To neutralize chemokines, ticks secrete small cysteine-rich chemokine-binding proteins in their saliva with no homologues in mammals, termed Evasins. In contrast to the highly selective Evasin-1, its homologue Evasin-4 binds ∼20 CC-chemokines with nanomolar affinity. Among this broad range of chemokines, the chemokine CC-motif ligand 5 (CCL5, also known as RANTES) is of particular interest, because it is one of the most expressed chemokines by activated platelets and plays a prominent role in the development of atherosclerosis. Thus, Evasin-4 binds to the CCL5 monomer and causes disruption of the CCL5 dimer by shifting the monomer/dimer equilibrium toward the monomeric form of the chemokine and not by direct replacing of CCL5 from the dimer.

In the present study, the structure of Evasin-4 was determined by X-ray crystallography. The Evasin-4 structure consists of eight β-strands and one short α-helix and has an L-shaped topology with the N- and C-terminal subdomains oriented orthogonally. Superposition of all six polypeptide chains of the three Evasin-4 crystal forms showed that the rigid Evasin-4 protein core is flanked by two more flexible protrusions. The first protrusion is formed by the N-terminal region (Glu16–Leu25) plus the loop β3–β4 (Ser48–Thr51) that extend from the N-terminal β-sheet. The second protrusion extends from the C-terminal β-sheet and consist of the loop β5–β6 (Asp68–Tyr82), including the α-helix (Ala74–Gln77). Residues Glu1–Glu15 are unresolved in all three crystal forms as a result of high flexibility. The crystal packing reveals a large intermolecular interface of 2,380 Å2 buried surface area common to all three Evasin-4 crystal forms. This interface involves the N-terminal region of Evasin-4 that forms an extended intermolecular antiparallel β-sheet, predominantly involving strand β1 next to strands β3 and β4 of each molecule. However, size-exclusion chromatography (SEC) and multiangle light scattering (MALS) analysis in solution show that Evasin-4 is a monomer, indicating that the packing in the crystal may not be physiologically relevant. In addition, the six independent structures of Evasin-4, arising from three different crystal forms we report here, are very similar to each other, suggesting that the crystal packing does not have major consequences on the overall structure of Evasin-4.

>[4x]EVPQMTSSSAPDLEEEDDYTAYAPLTCYFTNSTLGLLAPPNCSVLCNSTTTWFNETSPNNASCLLTVDFLTQDAILQENQPYNCSVGHCDNGTCAGPPRHAQCW>MGGGFAVNYNFDEIIDRRYTNAMNVEGYKGYLFGDADTSDLKDNDELIRMWVADMDFGTPEVVLNAIRERLNKKILGYTNVFGSEYYEAFVSWTKKRYGFTFSQEHLVFSHGIVAGLIELVGYICDKDDKALIVTPSYGPFKMACDKNHISTVYSPLINHHGYYEIDFDDVRKKVETENIKLCIFANPHNPTGRVWSEEELATLGQIMKENDVWLISDEIHCDIKRSGQSHIPFAKAVPDYDKIITTMSQSKAFNIAGLMFSNIIIQNESLLKTWNTHHFGTENPLSVVATQAAYEKGEGWLQAMNHYLDDNFNYLADFLEKELPHAEFKIPEATYLAWVDLSYYIKEKDIDESMAKFFIKNAGVIIEGAEQFVHNAEGHIRINIAVPREVMKKGLQKIKAALVENLYFQGHHHHHHHHHH[2x];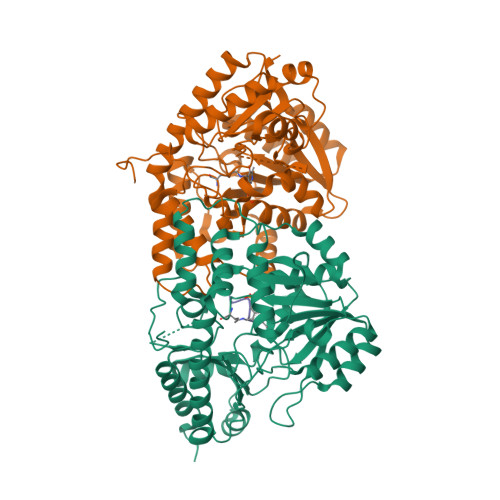> HHHHHH>MDLEYMHISYPNILL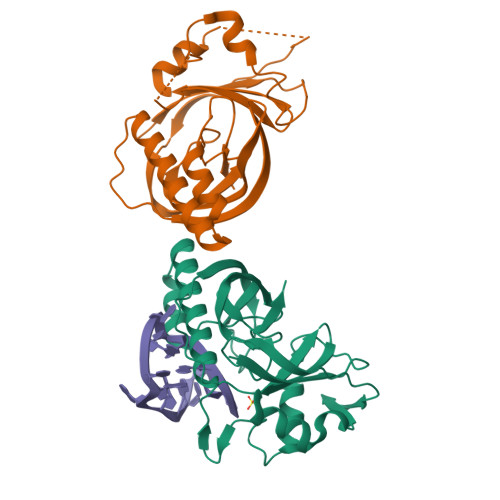NMRDGSKLRGYFAKKYIDEEIVHNHRDNAFVYKYPQIQFKIIDRSPLIIGIGSLGINFLESKRIFFEKELIISNDTNDITEVNVHKDMDHFGTTDKILKYQFKTPWMALNAKNSEIYKNSDEIDREEFLKRVLIGNILSMSKSLGYTIEEKLKVKINLKEVPVKFKNQNMVGFRGEFYINFDIPQYLGIGRNVSRGFGTVVKV[6x]>[3x]MAQILPIRFQEHLQLQNLGINPANIGFSTLTMESDKFICIREKVGEQAQVVIIDMNDPSNPIRRPISADSAIMNPASKVIALKAGKTLQIFNIEMKSKMKAHTMTDDVTFWKWISLNTVALVTDNAVYHWSMEGESQPVKMFD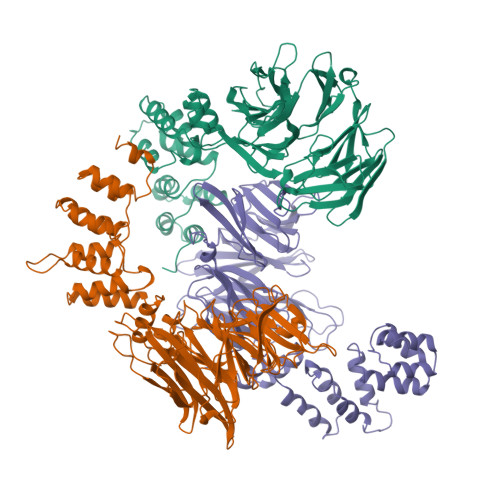RHSSLAGCQIINYRTDAKQKWLLLTGISAQQNRVVGAMQLYSVDRKVSQPIEGHAASFAQFKMEGNAEESTLFCFAVRGQAGGKLHIIEVGTPPTGNQPFPKKAVDVFFPPEAQNDFPVAMQISEKHDVVFLITKYGYIHLYDLETGTCIYMNRISGETIFVTAPHEATAGIIGVNRKGQVLSVCVEEENIIPYITNVLQNPDLALRMAVRNNLAGAEELFARKFNALFAQGNYSEAAKVAANAPKGILRTPDTIRRFQSVPAQPGQTSPLLQYFGILLDQGQLNKYESLELCRPVLQQGRKQLLEKWLKEDKLECSEELGDLVKSVDPTLALSVYLRANVPNKVIQCFAE>MGSLVCVGTGLQLAGQISVLSRSYIEHADIVFSLLPDGFSQRWLTKLNPNVINLQQFYAQNGEVKNRRDTYEQMVNAILDAVRAGKKTVCALYGHPGVFACVSHMAITRAKAEGFSAKMEPGISAEACLWADLGIDPGNSGHQSFEASQFMFFNHVPDPTTHLLLWQIAIAGEHTLTQFHTSSDRLQILVEQLNQWYPLDHEVVIYEAANLPIQAPRIERLPLANLPQAHLMPISTLLIPPAKKLEYNYAILAKLGIGPEDLG[2x];>[2x]MSGLSD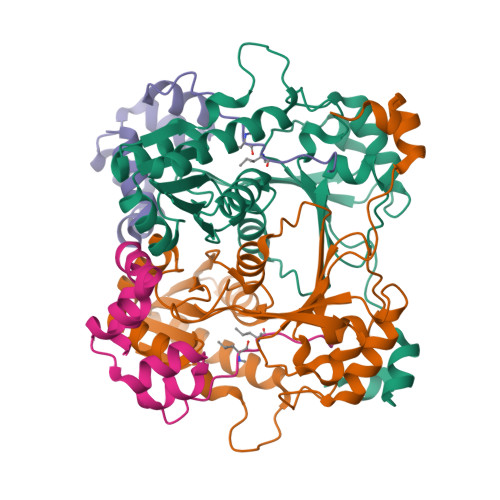FFTQLGQDAQLMEDYKQNPEAVMRAHGLTDEQINAVMTGDMEKLKTLSGDSSYQSYLVISHGNGD quinazolin-2-amine | C8 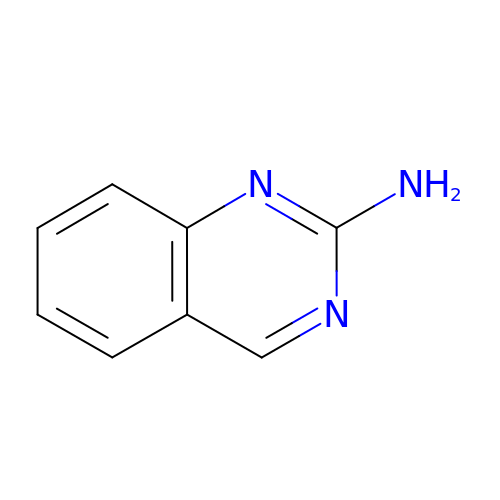H7 N3 | CZAAKPFIWJXPQT-UHFFFAOYSA-N>AKTKAAVSMEGFSWGNYINSNSFIAAPVTCFKHAPMGTCWGDISENVRVEVPNTDCSLPTKVFWIAGIVKLAGYNALLRYEGFENDSGLDFWCNICGSDIHPVGWCAASGKPLVPPRTIQHKYTNWKAFLVKRLTGAKTLPPDFSQKVSESMQYPFKPCMRVEVVDKRHLCRTRVAVVESVIGGRLRLVYEESEDRTDDFWCHMHSPLIHHIGWSRSIGHRFKRSDITKKQDGHFDTPPHLFAKVKEVDQSGEWFKEGMKLEAIDPLNLSTICVATIRKVLADGFLMIGIDGSEAADGSDWFCYHATSPSIFPVGFCEINMIELTPPR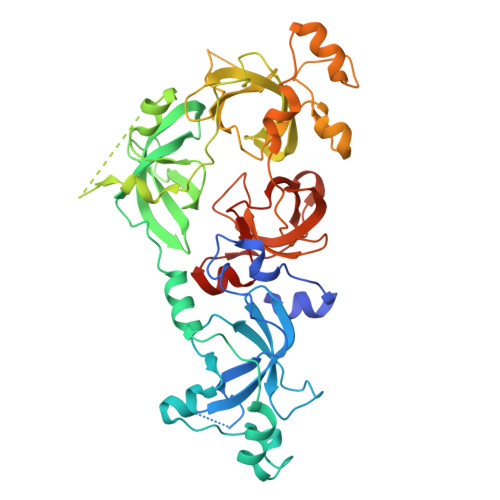GYTKLPFKWFDYLRETGSIAAPVKLFNKDVPNHGFRVGMKLEAVDLMEPRLICVATVTRIIHRLLRIHFDGWEEEYDQWVDCESPDLYPVGWCQLTGYQLQPPASQSSR[2x]> MASMTGGQQMGRDEAGITGTWYNQLGSTFIVTAGADGALTGTYESAVGNAESRYVLTGRYDSAPATDGSGTALGWTVAWKNNYRNAHSATTWSGQYVGGAEARINTQWLLTMGTTEANAWASTLVGHDTFTKVKPSAASIDAAKKAGVNNGNPLDAVQQ

ArMs consist of an organometallic moiety anchored within a protein scaffold thereby combining some of the most attractive features of both homogeneous catalysis and biocatalysis. The biotin-streptavidin technology ranks amongst the most versatile platforms for the generation of ArMs. Herein we present an E. coli surface display platform for streptavidin (Sav hereafter) relying on an Lpp-OmpA anchor. The system was used for the high throughput screening of a bioorthogonal CpRu-based artificial deallylase (ADAse) that uncages an allylcarbamate-protected aminocoumarin 1.

Two rounds of directed evolution afforded the double mutant S112M–K121A that displayed a 36-fold increase in surface activity vs. cellular background and a 5.7-fold increased in vitro activity compared to the wild type enzyme. To our delight, [CpRu(QA-Biot)(OH2)] 3·Sav-S112M–K121A afforded high resolution diffraction data. The crystals were obtained by sitting drop vapor diffusion, followed by soaking with cofactor [CpRu(QA-Biot)(OH2)] 3 and flash freezing in liquid nitrogen (see ESI†). The [CpRu(QA-Biot)(OH2)] 3 cofactor was modeled with 100% occupancy within the Sav biotin binding site (Fig. 3c and S21†). The piperazine linker and the ruthenium carboxyquinoline moiety are localized in a single conformation within the biotin vestibule. The aromatic quinoline ring is stabilized by a methionine–π interaction with the neighboring S112M side chain. The aliphatic side chains of L124 and L124* (* indicates the neighboring Sav monomer) and the carbonyl moieties of residues K121A and S122 form a pocket that harbors the quinoline ligand. Spherically-shaped electron density around the ruthenium suggests that the cofactor may exist as a mixture of epimers (i.e. (R)- and (S)-Ru). The Cp and water ligands were thus not modeled due to the ambiguity of the electron density. X-ray crystallography of ADAse double mutant S112M–K121A highlights the localization of cofactor 3 within the biotin-binding vestibule.> MAMVINVSFKVTGGKEFTVAIEPDITVLDLKKICAEHVDIPVEAQRIIFKG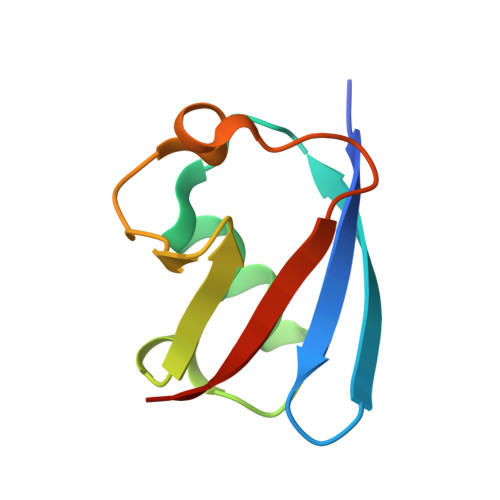KILKDKESLTLYGVADGNTMHLVRSAMA>MTINYQFGDVDAHGAMIRAQAGLLEAEHQAIVRDVLAAGDFWGGAGSVACQEFITQLGRNFQVIYEQANAHGQKVQAAGNNMAQTDSAVGSSWATHHHHHH[2x];>[2x]SMATRFMTDPHAMRDMAGRFEVHAQTVEDEARRMWASAQNISGAGWSGMAEATSLDTMAQMNQAFRNIVNMLHGVRDGLVRDANNYEQQEQASQQILSS

Of particular interest are the Esx complexes which are dimers of two subunits (ESAT-6, early secreted antigen of 6 kDa; and CFP-10, culture filtrate protein of 10 kDa) and which are secreted across the cytoplasmic membrane by Type VII secretion (T7S) systems. Mycobacterial ESX secretion systems have been shown to be involved in a variety of physiological processes including conjugation in a non-pathogenic mycobacterium, iron and/or zinc acquisition by both pathogenic and non-pathogenic mycobacterial species, and virulence of pathogenic mycobacteria. The overall architecture of the complexes is similar to known Esx structures in that each heterodimer forms a four helix bundle with the CFP-10 and ESAT-6 subunit homologs each contributing an α-helical hairpin to the complex. The subunit interfaces in the four-helix bundles of the Esx complexes are similar to those of the previously determined Esx complex structures in that the intermolecular interface between the CFP-10 and ESAT-6 subunits is largely hydrophobic.

A crude low resolution model of the SeMet-labeled EsxEFma complex was used to obtain a molecular replacement solution for a high resolution (1.96 Å) EsxEFma native dataset and a second crystal form of EsxOPmt, solved by molecular replacement using the EsxOPmt model from form I, at 2.55 Å was also obtained. The asymmetric units for the EsxEFma crystal forms have a single complex in the asymmetric unit for the SeMet-labeled protein and six complexes in the asymmetric unit of the native protein crystal form while the EsxGHms and EsxOPmt (both crystal forms) contain two heterodimeric complexes. The WXG-containing loops are well ordered in the EsxGHms complexes and in most of the EsxEFma complexes but the majority of the connecting loops are disordered in the EsxOPmt subunit structures. Additional regions of disorder are found at the N- and C-termini of the complexes with the EsxFma and EsxOmt subunits having a substantial number of disordered residues at their C-termini. The average amount of buried surface area in the subunit interfaces varies considerably [EsxEFma, ∼1605 Å2; EsxGHms, ∼1555 Å2; EsxOPmt (form I), ∼1025 Å2; and EsxOPmt (form II), ∼1175 Å2] and the percentage of the surface of each subunit buried in the complex interface is also highly variable, from 13.5–33%, and is related to the degree to which the termini of the subunits are ordered and to the conformations that they adopt. Shape complementarity (Sc) statistics of 0.77 for EsxEFma, 0.74 for EsxGHms, and 0.69 and 0.71 for EsxOPmt forms I and II, respectively, indicate that the interfaces are highly complementary, with biologically significant interfaces such as antibody-antigen interactions generally having values in the range of 0.65–0.85.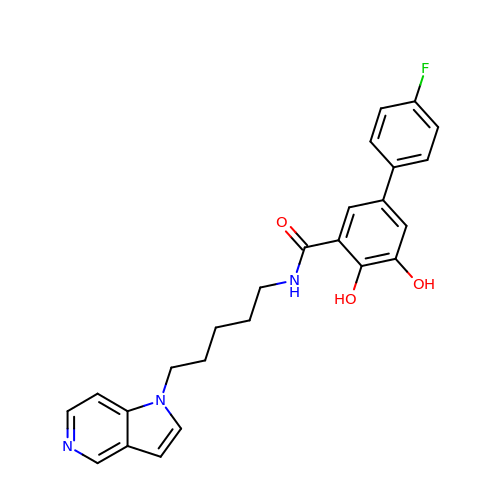5-(4-fluorophenyl)-2,3-dihydroxy-N-(5-pyrrolo[3,2-c]pyridin-1-ylpentyl)benzamide | C25 H24 F N3 O3 | IPHKDWUCDYFNGH-UHFFFAOYSA-N>GPLGSDLITCYCRKPFAGRPMIECSLCGTWIHLSCAKIKKTNVPDFFYCQKCKELRPEARR[5x]

In the NUP98–PHF23 chimera, the amino-terminal portion of NUP98 with multiple GLFG repeats is fused to the carboxy-terminal portion of PHF23 that contains a single PHD finger (PHF23PHD). In this study, we report molecular mechanisms for the recognition of methylated histone H3K4 by the PHD finger of PHF23 and inhibition of this interaction by small molecule compounds DS and amiodarone (AD). In contrast, H3K4me1 and H3K4me0 peptides induced CSP in PHF23PHD in fast exchange regime, and plotting these resonance changes against peptide concentration yielded Kds of 580 μM and 1.6 mM, respectively. These results suggest that PHF23PHD selects for the higher methylation state of H3K4 (tri- and dimethylated) and discriminates against monomethylated (H3K4me1) or unmodified H3. Collectively, our data indicate an overall similar mode of action for these NUP98 fusions during AML development that depends on binding of their PHD fingers to H3K4me3, a mark enriched at promoters of actively transcribed genes.

To better understand the mechanism by which PHF23PHD recognizes the histone tail, we determined the protein structure. Although PHF23PHD was crystallized in the presence of H3K4me3 peptide, unexpectedly we obtained the structure in which the N-terminal sequence of one PHF23PHD molecule was bound to the second PHF23PHD molecule. Alignment of this structure with the structures of other PHD fingers, such as of KDM5A and BPTF in complex with H3K4me3 peptides (see discussion below), revealed that the N-terminal sequence DLIT (residues 338–341 of PHF23PHD) and a preceding serine derived from the vector superimpose very well with H3K4me3 in the KDM5A and BPTF complexes. Much like H3K4me3, the SDLIT sequence is bound in an extended conformation and pairs with the β1 strand of PHF23PHD, which results in the formation of the three-stranded antiparallel β-sheet. The I340 side chain occupies the aromatic/hydrophobic cage of PHF23PHD consisting of F348, M353, and W362 with another hydrophobic residue, L339 being positioned to make an additional wall of the cage. Mapping the most perturbed residues of the protein (due to binding of H3K4me3) on the surface of PHF23PHD confirmed that H3K4me3 occupies the same binding pocket of PHF23PHD as the SDLIT sequence. Of note, I340 in the SDLIT sequence superimposes well with the hydrophobic part of the K4me3 side chain, further suggesting that lysine mimetics could also occupy the aromatic cage. Substitution of either M353 with valine or W362 with alanine abolished the interaction with H3K4me3, and replacement of F348 with alanine led to protein unfolding, suggesting a role of this residue in structural stability of PHF23PHD.> SSGDSSRNKVKETLRLFHGVCRKILQEDEAKPEDQRRKGKGLRIDFEASTILKRNGKFLNSGVHILGEVPGVEVGDEFQYRMELNILGIHKPSQAGIDYMKYGKAKVATSIVASGGYDDHLDNSDVLTYTGQ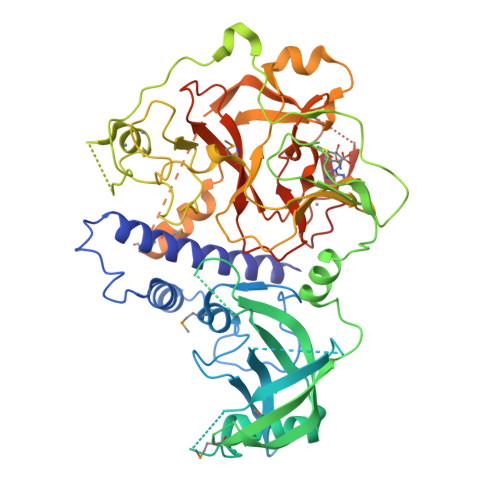GGNVMQVKKKGEELKEPEDQKLITGNLALATSIEKQTPVRVIRGKHKSTHDKSKGGNYVYDGLYLVEKYWQQVGSHGMNVFKFQLRRIPGQPELSWVEVKKSKSKYREGLCKLDISEGKEQSPISAVNEIDDEKPPLFTYTVKLIYPDWCRPVPPKSCCCTTRCTEAEARVCACVEKNGGEIPYNFDGAIVGAKPTIYECGPLCKCPSSCYLRVTQHGIKLPLEIFKTKSRGWGVRCLKSIPIGSFICEYVGELLEDSEAERRIGNDEYLFDIGNRYDNSLAQGMSELMLGTQAGRSMAEGDESSGFTIDAASKGNVGRFINHSCSPNLYAQNVLYDHEDSRIPHVMFFAQDNIPPLQELCYDYNYALDQVRDSKGNIKQKLCFCGAAVCRRRLY> ALFDSLLARN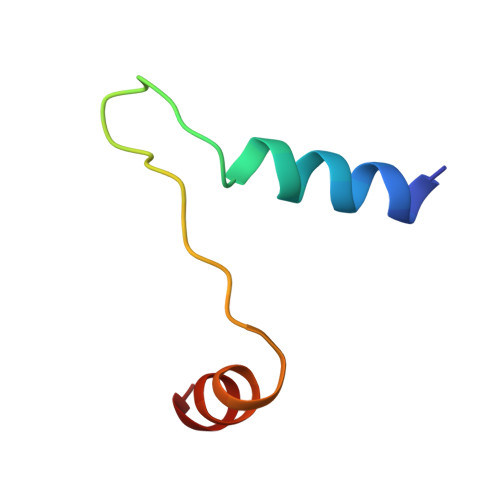KKQAEGETALGELPSLQLGLADLRQRLRKL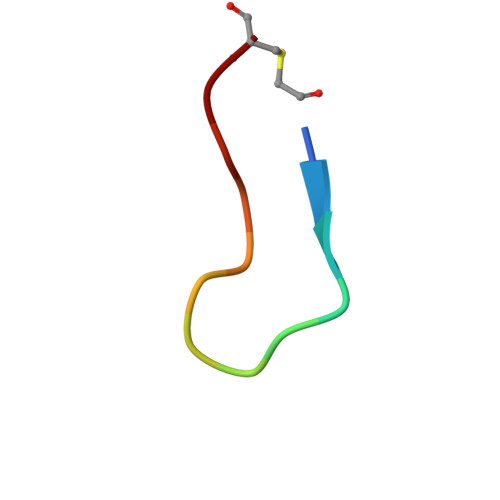> FITGHYWVRFLPC> MAQTFEGTLQSLLQGVSQQIPRERQPGQLGAQQNMLSDPVTGLRRRPPLHLAAQTLMENPVSPDALFS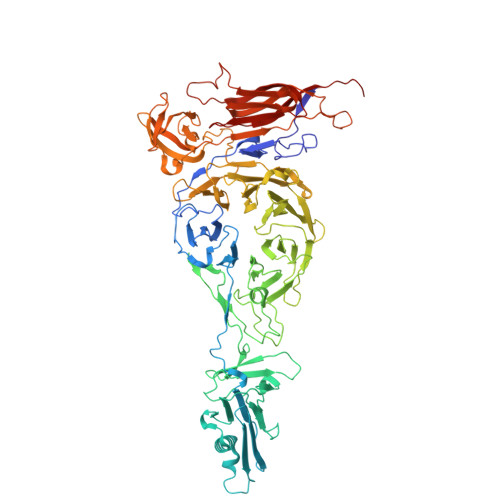TYIERGTDGRHLLINTEAGIWQILSKDATTLIRSGQADYLKASIGATSIQTASIAGLTYILNTEQTPVAHVDNTGKLNPANTGFFYIVASSFSKRWTITVQSNEGTWTAVHDVGASSDDGAVPAATASAVINSLKTNLLAAGMPSDKVDTFGSYMFIKGLTNVVVSSDAGTTYARWSNQSRVDEESDLPAQLPASANGCMCRVGAASTSATWYRFDYATRQWNEDSAYSSITKITNMPLEFAADDQIIPRDFEGRLAGDDENNEDPGFVENGYITGIAAFQGRLVLLSGSRVSMSASGLYQRFYRSTVVNLLDTDRIDIGAASAQDSVFRAALQFNRDLVVFGDSMQAVIAGNAVLTPTNASIALTSEFSCDSRVIPVVTGQTVLYASRRNSDYAGLLEFIPSAYTSSQYVSQDATVHLPRYIPGRVMDMQVSSVTNVAFFRYSGERTSVLVYEFLWGEDAKRAQGAYHKWVLPYDVLSLHTLSEAAYFFVRGPGAYVLALRVDPREGFVAGTTYEYPFMDMGAPVTVQGGQFTLPEHLRKAGLQDSIALAYYTGDDSGSELGIASISSNWVCTTVRGVPDGNYLAGYRFKSGTTLTPPMLKDQNDNLIGSGHVRLLRLDVAMRNSGVVDVLVEDNARDVDNDSEYSGVLMNSKELAPEQPLKASLSNIIIPCRTNTDTTEVTLSTSGTLEMNIMDVSYILRYNQRRRRV> GSAMGSKAVDDTKEALAGGKILHNQNVNDWERVVVTPTADGGESRFDGQIIVQMENDDVVAKAAANLAGKHPESSVVVQIDSDGNYRVVYGDPSKLDGKLRWQLVGHGRDDSESNNTRLSGYSADELAVKLAKFQQSFNQAENINNKPDHISIVGASLVSDDKQKGFGHQFINAMDANGLRVDVSVRSSELAVDEAGRKHTKDANGDWVQKAENNKVSLSWDEQG

V. vulnificus secretes a large multifunctional-autoprocessing repeats-in-toxin (MARTX) as a main virulence factor via an atypical type I secretion system. The central region of the MARTX toxin of V. vulnificus MO6-24/O contains an autoprocessing cysteine protease domain (CPD) and four effector domains including the domain of unknown function (DUF1), the Rho-inactivating domain (RID), an αβ hydrolase (ABH), and makes caterpillars floppy-like domain (MCF). The CPD directs the proteolytic processing of effector modules after activation by binding to the eukaryotic cell-specific inositol hexakisphosphate (InsP6). The V. vulnificus MARTX CPD displays a canonical CPD structure with the central seven-stranded β-sheet flanked by three α helices.

To examine the activated conformation of the unprocessed CPD upon InsP6-binding, we crystallized the pre-processing form of CPD (here referred to as pre-CPD) bound to InsP6 using the catalytically inactive mutant C3727A. We determined the 1.3Å crystal structure of the CPD-InsP6 complex capturing the scissile bond harbored in the active site. The N-terminal five residues (TKEAL, 3583–3587) upstream of the scissile bond were ordered in the crystal structure. The side chain of the scissile residue Leu3587 is inserted into the catalytic pocket formed between catalytic residues His3678 and Cys3727. The Cβ atom of the mutated Cys3727Ala points toward the amide bond of the scissile bond, which represents the conformation ready for the catalytic reaction. The backbone of Leu3762 in β9 makes a hydrogen bond with the amide nitrogen of the scissile residue Leu3587. InsP6 binds to the conserved basic pocket located distal to the substrate binding pocket. Three positively charged residues, Arg3769, Lys3770, and Lys3782 of the β-flap make ionic interactions with InsP6. The β8-β9 loop of the β-flap interacts with the β7-α3 loop locking the catalytic residue Cys3727 in an active conformation. The binding affinity of InsP6 to the pre-CPD C3727A was 1.4 ± 0.5 μM measured by isothermal titration calorimetry.> KPVVGVILPFSSAFEDIAVEQQRAVELALAESGSAFEIVFKDGGADVDTAVQAFQDLVRSQENLAAVVSCSSWASSAIHPLAAEKDIFHVAIGSAALKRTEPGHTIRLTVGVQQEQEQLAAYLTDFERIAVLAMDNNLGSSWIRMLEDRFPKQVVAAQEYNPQQMDIAAQLATIKARDSEALVLISAGEAATIAKQARQAGIKAQLVGTRPIQRAEVLAASAFTNGLVYTYPSYNQDHPFMSAFTDRYGLEPGFFGVEAYDLCTTLSRALEQGR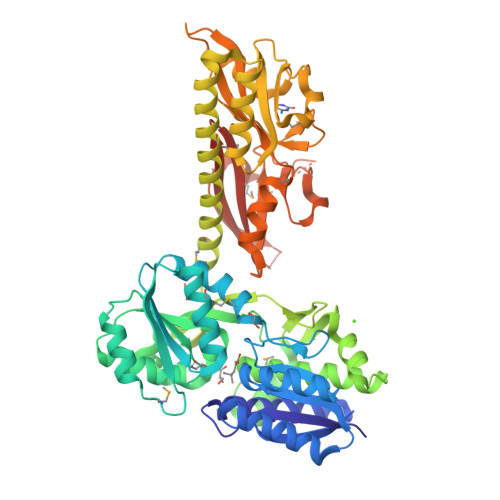QTPKALFEWYAGNTFTGALGKVTFANDGDASYPYIFKKVTESGFRVAEFQFPMLLTQTAQELNAIFKDMDRSVAAAAEQLSTTGLRGDRASAILETLFNENQYAYNCVTVDATGTIVNVAPKQYSSVIGEDISGQEQIIRLHETHQPVLSQAIKMVEGFVGIDLEHPVFDQDGGFIGSVSVLTQPDFFGSIISRKVHNFPVEIFVLQRDGTTIYDVNAEEIGKNAFADPIYDAFPSLKRIARKMVSQAEGEGTYRFQDRHMEHAVAKQLLWTSIGLHGTNYRLALTYGAGEIED>[12x]MSEMTPREIVSELDQHIIGQADAKRAVAIALRNRWRRMQLQEPLRHEVTPKNILMIGPTGVGKTEIARRLAKLANAPFIKVEATKFTEVGYVGKEVDSIIRDLTDSAMKLVRQQEIAKNRARAEDVAEERILDALLPPAKNQWGEVENHDSHSSTRQAFRKKLREGQLDDKEIEIDVSAGVSMGVEIMAPPGMEEMTNQLQSLFQNLGSDKTKKRKMKIKDALKALIDDEAAKLINPEELKQKAIDAVEQNGIVFIDEIDKICKKGEYSGADVSREGVQRDLLPLVEGSTVSTK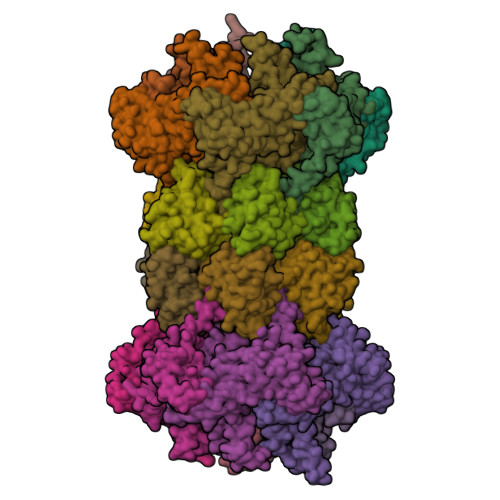HGMVKTDHILFIASGAFQVARPSDLIPELQGRLPIRVELTALSAADFERILTEPHASLTEQYKALMATEGVNIAFTTDAVKKIAEAAFRVNEKTENIGARRLHTVMERLMDKISFSASDMNGQTVNIDAAYVADALGEVVENEDLSRFIL;>[12x]TTIVSVRRNGQVVVGGDGQVSLGNTVMKGNARKVRRLYNGKVLAGFAGGTADAFTLFELFERKLEMHQGHLLKSAVELAKDWRTDRALRKLEAMLIVADEKESLIITGIGDVVQPEEDQILAIGSGGNYALSAARALVENTELSAHEIVEKSLRIAGDICVFTNTNFTIEELPN A deazaflavin-dependent nitroreductase (Ddn) from Mycobacterium tuberculosis catalyzes the reduction of nitroimidazoles such as PA-824, resulting in intracellular release of lethal reactive nitrogen species. The N-terminal 30 residues of Ddn are functionally important but are flexible or access multiple conformations, preventing structural characterization of the full-length, enzymatically active enzyme. The split barrel-like fold is characterized by a central six-stranded antiparallel β barrel in a Greek key topology with four α helices: A at the N terminus (the putative helix removed for Ddn structure determination), B after an extended loop between strands β3 and β4, and C and D between strands β5 and β6. The identification of these residues and the lack of classic catalytic residues in the active site suggest that Ddn functions primarily by precisely orienting PA-824 for efficient direct hydride transfer from F420 and potentially through additional transition-state stabilization.

In order to characterize a full-length enzyme including the N terminus, we also determined the structure of nfa33440, a homolog from N. farcinica sharing 42% sequence identity to Ddn and that was active in the PA-824 in vitro assay. The structure of this protein was solved by molecular replacement using the Ddn structure. Although an initial apo structure lacked density for the first 37 amino acids, a cocrystal of nfa33440 with F420 confirmed that the overall structure and coenzyme binding are very similar to that of Ddn (rmsd is 0.95 Å over 109 aligned Cα atoms to Holo-1). The N terminus of nfa33440 is represented in the electron density starting at residue 6, showing an extended sequence packed against the core of the protein followed by a short α helix flanking the F420 binding site. Although interpretation is uncertain without assigning the spectrum, these data, along with the lack of density for the N terminus in the apo-nfa33440 crystal, suggest that nfa33440 in solution consists of a structured core with the N terminus undergoing conformational exchange processes similar to the Ddn mutants. In the lowest-energy model, the nitroimidazole group of PA-824 is located near the Re face of F420, with the nitro group H bonded with the side chains of S78, Y130, and Y136. Notably, S78 in Ddn and S72 in nfa33440 are bound to a water modeled near some chains of the crystal structures (shown for Holo-1, chain E in Figure 3D), which may mimic binding to one oxygen atom of the nitro group of PA-824. Mutation of S78 (nfa33440 S72) resulted in loss of activity, as did perturbation of nearby residues likely to help position S78 (Ddn R142, I144; nfa33440 R136, I138). The proposed role of the Ddn Y130 (nfa33440 Y124) hydroxyl for substrate binding and orientation was also substantiated because mutation of Tyr to Phe significantly lowered catalytic competence in either enzyme.

>[4x]GMRMSSTGEYVPSPSEWIGNQVAQYEASDGAEAGEFDGRPLVILTTVGRKTGALRKTPVMRVEHDGRYAVVASQGGAPTHPAWYFNLVADPRAQLRDKDAVLSVVARELAGPERAEWWERAVRAYPTYQEYQDNTRRLIPVLLLEPG N-[2-(dimethylamino)ethyl]-2-methyl-2-[4-[4-[[2-methyl-5-[(2S,3R,4R,5S,6R)-6-methylsulfanyl-3,4,5-tris(oxidanyl)oxan-2-yl]phenyl]methyl]phenyl]butanoylamino]propanamide 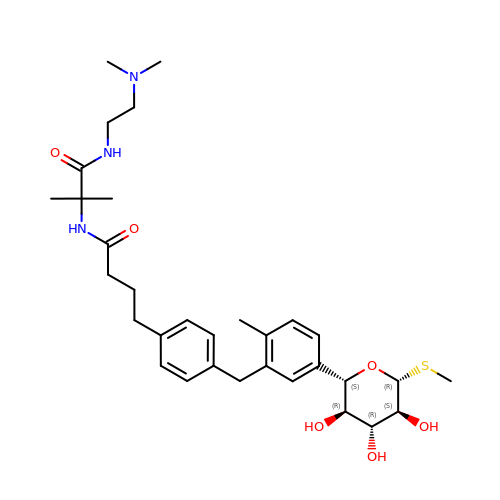| C32 H47 N3 O6 S | BNPZTRDIESRGTC-IXYVTWBDSA-N> LNIDMNWLGQLLGSDWEIFPAGGATGDAYYAKHNGQQLFLKRNSSPFLAVLSAEGIVPKLVWTKRMENGDVITAQHWMTGRELKPKDMSGRPVAELLRKIHTSKALLDMLKRLGKEPLNPGALLSQLKQAVFAVQQSSPLIQEGIKYLEEHLHEVHFGEK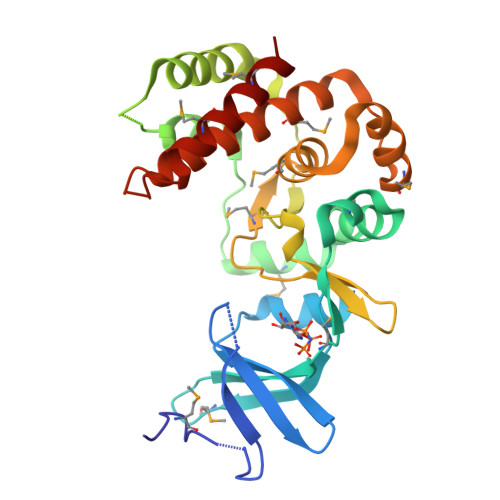VVCHCDVNHNNWLLSEDNQLYLIDWDGAMIADPAMDLGPLLYHYVEKPAWESWLSMYGIELTESLRLRMAWYVLSETITFIAWHKAKGNDKEFHDAMEELHILMKRIVD>SMSMKATRLAIPDVILFEPRVFGDDRGFFFES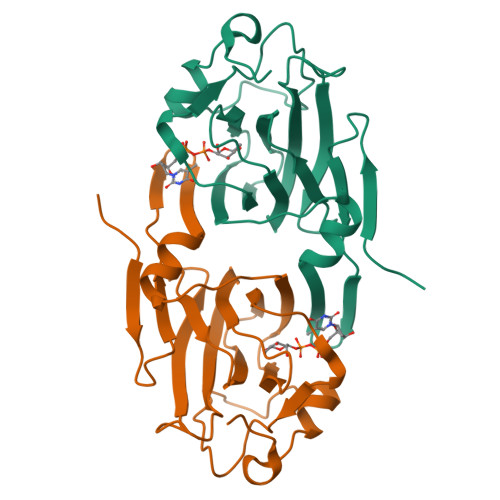YNQRAFEEACGHPVSFVQDNHSRSARGVLRGLHYQIRQAQGKLVRATLGEVFDVAVDLRRGSPTFGQWVGERLSAENKRQMWIPAGFAHGFVVLSEYAEFLYKTTDFWAPEHERCIVWNDPELKIDWPLQDAPLLSEKDRQGKAFADADCFP[2x]> ADPHKCDITLQEIIKT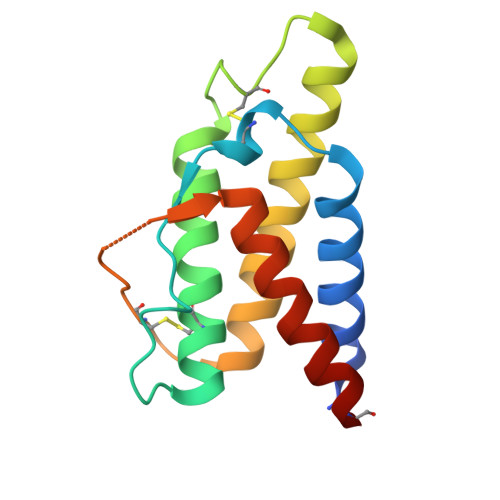LNSLTEQKTLCTELTVTDIFAASKNTTEKETFCRAATVLRQFYSHHEKDTRCLGATAQQFHRHKQLIRFLKRLDRNLWGLAGLNSCPVKEANQSTLENFLERLRVIMQSKWFKCGA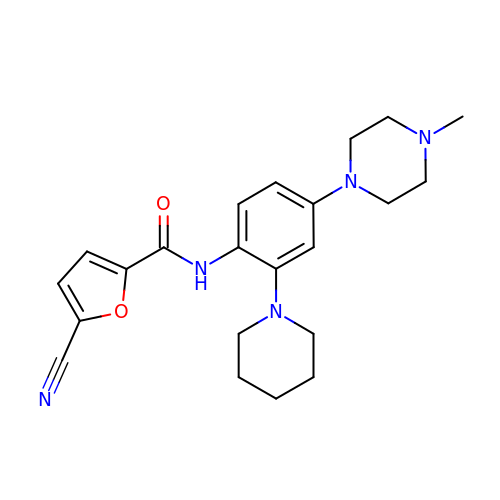5-cyano-N-[4-(4-methylpiperazin-1-yl)-2-piperidin-1-ylphenyl]furan-2-carboxamide | C22 H27 N5 O2 | UUPPIQKPNBIUKY-UHFFFAOYSA-N> MHHHHHHSPLRVALYGFGNQNKEMAKMLVERKDVEIVAVISNKSNVGKDFGEVIGLAPQGILVTAGLDAAETLRTTNPQIAMLSTLSTVGDIESQLRACAENKVNVYTIAEELTFSWTSAPEKTKEMDELFKEHNVSLIGGGFLDGACCDMARTMAAMMHKIDKLDGGLQYNVDHYGQVLAIAHGVGLSEEEFYAENGPGWTSPTSYPKSYVYNMNDWFASAFG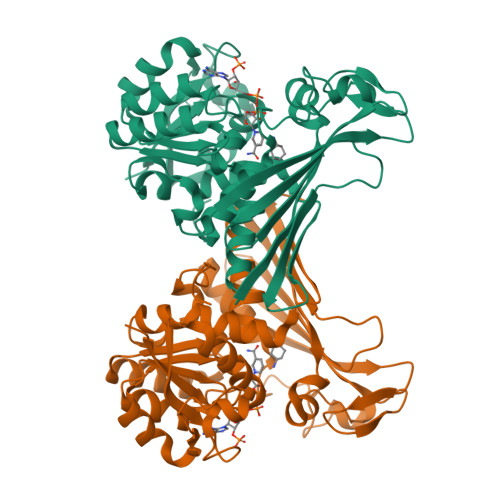LTVIKTEEVKTPTKAPIELYSEAIGRAIPVGQCTGMIVTATTTTEEGVIIVEKQVGKCYEDGDEDMVFMNLEGNPTGGVGFTMKNPPTPAMTNTIAISRMFQTVDAPAGYITTDKLPTMEAYVHGRL>CRQKGAGSAGTGSETNSQEVRSQMRSTCLIIPKERFRTMAKEISKKEGHDVHIAEAALDMLQVIVESCTVRLLEKALVITYSGKRTRVTSKDIETAFMLEHGPLLE[2x];>[2x]LADHVSVGETQIPKASTQHLLRKAGSLSAAGDTEVPIRGFVHMKLHKLVQKSLLAMQLAKRKTIMKSDVKKAAELMHLPVFAIPTKDSGAKGSVFLS;> ESKEGSRSSKAKLQISVARSERLLREHGGCSRVSEGAAVALAAAIEYFMGEVLELAGNAARDSKKVRISVKHITLAIQNDAALFAVVGKGVFSGAGVSLISVPIPRKKARKTTEKEASSPKKKAAPKKKKAASK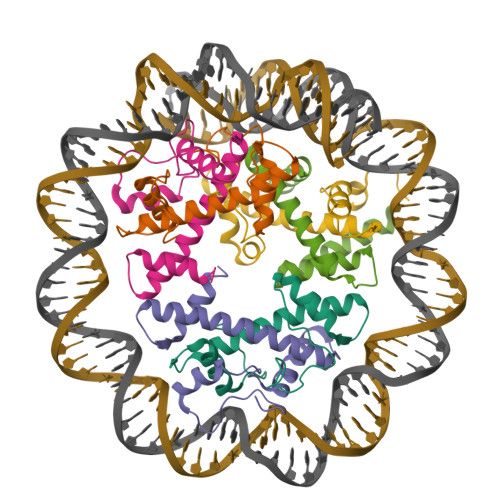QKKSLSDKELAKLTKKELAKYEKEQGMSPGY;> MATQKETTRKRDKSVNFRLGLRNMLAQIHPDISVQTEALSELSNIAVFLGKKISHGAVTLLPEGTKTIKSSAVLLAAGDLYGKDLGRHAVGEMTKAVTRYGSAK> LPISMSDEGDSFLVKDSLGENKIPKNPSKVVILDLGILDTFDALKLNDKVVGVPAKNLPKYLQQFKNKPSVGGVQQVDFEAINALKPDLIIISGRQSKFYDKLKEIAPTLFVGLDNANFLSSFENNVLSVAKLYGLEKEALEKI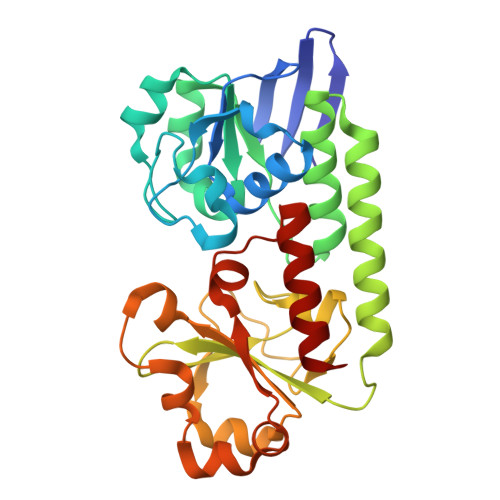SDIKNEIEKAKSIVDEDKKALIILTNSNKISAFGPQSRFGIIHDVLGINAVDENIKVGTHGKSINSEFILEKNPDYIFVVDRNVILGNKERAQGILDNALVAKTKAAQNKKIIYLDPEYWYLASGNGLESLKTMILEIKNAVK> MLNPNRIKDEFSVRLEDIENSINESYNLSTIGGDFAAIATDDAVFESYKDQLLEGFDAAEGEALAGMLDNTREEILMESSMGPIQPYASLSMPILVKLWARLALTEALPTQVANKPNFTVPILTPYVVDADGNKHALPESINNTPETLVGLVQIKEDIAVEGGKVTDYDLFTGLKEGKEVRKGIDRLDRKFKIVEAKWSDSFDERTSAAGFVELGSNVVKLQDNDTLVGQIKYPTNGDGEVETDTILGKVDVSSGELTLTSASGKLTDVKVKGYVASEQHTSATNVELGLTRKDVVIDTAQHIEATVPLEVIQDMKATYDIDGVARLSETMSQLSSQKVDLDIIEFLDHEYKETDAKYHFSFDVFPHSDYSAHPKDWLEGLREVIDHTTQSMKNDYKLYDVQFVIVGNPLDVRLIPNVSWTFNGGDRNADAYSNGIKINYSLGAASGTANYRIIGSDLVRQGELTIIAIPQQDNYKTFMFYPYTFNVVNGG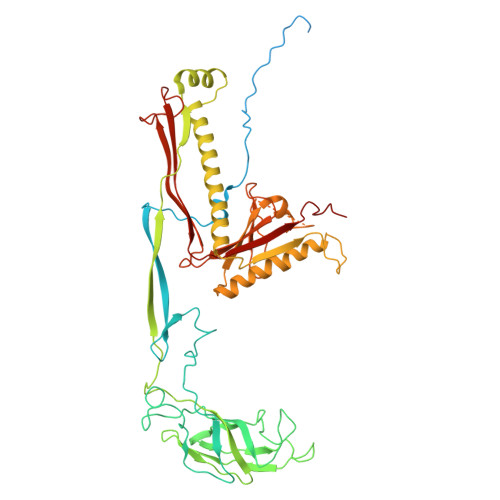GYLNTRNPNVPNMMMTRRYTVESFVPIIGRITIKNNNGSVYAR>[2x]MHHHHHHADLAESNIKVMCRFRPLNESEVNRGDKYIAKFQGEDTVVIASKPYAFDRVFQSSTSQEQVYNDAAKKIVKDVLEGYNGTIFAYGQTSSGKTHTMEGKLHDPEGMGIIPRIVQDIFNYIYSMDENLEFHIKVSYFEIYLDKIRDLLDVSKTNLSVHEDKNRVPYVKG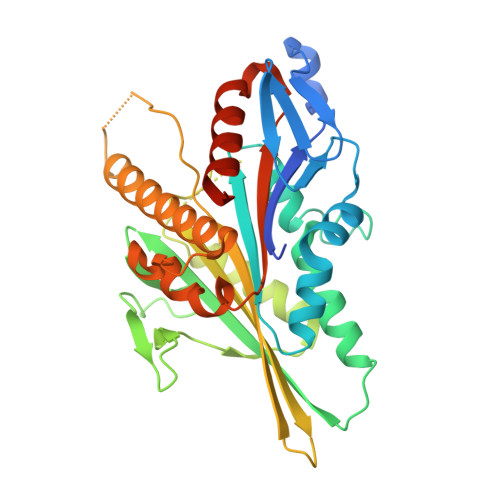ATERFVSSPDEVMDTIDEGKSNRHVAVTNMNEHSSRSHSIFLINVKQENTQTEQKLSGKLYLVDLAASEKVSKTGAEGAVLDEAKNINKSLSALGNVISALAEGSTYVPYRDSKMTRILQDSLGGNARTTIVICCSPSSYNESETKSTLLFGQRAKTIKNTVSVNVELT>[3x]MGSKDGTGDI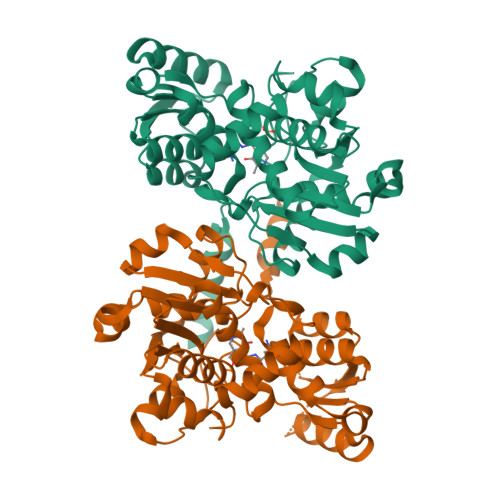SEAQGYAADIDSIREAQARIAPYVHRTPVMSSTSIDAMVGKKLFFKCECFQKAGAFKIRGASNSIFALDDEQVSKGVVTHSSGNHAAAVALAAKLRGIPAHIVIPRNAPASKVENVKCYGGHIIWSDASIESREYVSKRVQEETGAVLIHPINSKYTISGQGTVSLELLEQVPEIDTIIVPISGGGLISGVALAAKAINPSIRILAAEPKGADDSAQSKAAGKIITLPSTNTIADGLRAFLGDLTWPVVRDLVDDVIVVDDTAIVDAMKMCYEILKVAVEPSGAIGLAAALSDEFKQSSAWHESSKIGIIVSGGNVDLGTLWQSMYKHLEHHHHHH> ANPLYQKHIISINDLSRDDLNLVLATAAKLKANPQPELLKHKVIASCFFEASTRTRLSFETSMHRLGASVVGFSDSANTSLGKKGETLADT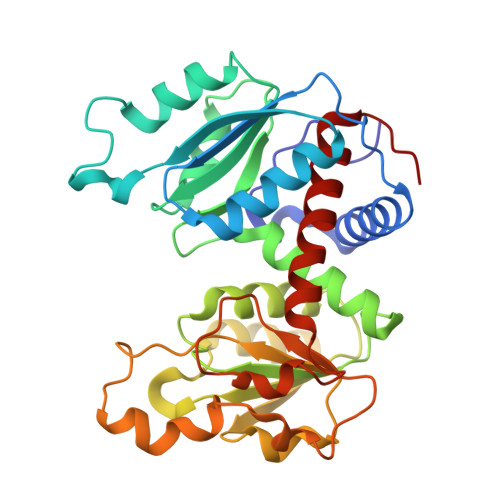ISVISTYVDAIVMRHPQEGAARLATEFSGNVPVLNAGDGSNQHPTQTLLDLFTIQETQGRLDNLHVAMVGDLEYGRTVHSLTQALAKFDGNRFYFIAPDALAMPQYILDMLDEKGIAWSLHSSIEEVMAEVDILYMTRVQKERLDPSKYANVKAQFVLRASDLHNAKANMKVLHPLPRVDEIATDVDKTPHAWYFQQAGNGIFARQALLALVLNRDLVL> MNQIWLKVCAASDMQPGTIRRVNRVGA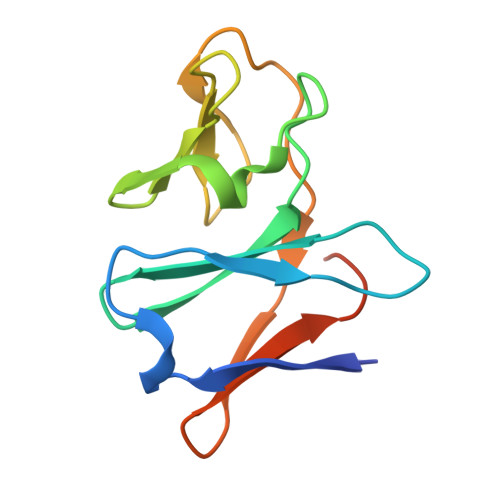APLAVYRVGDQFYATEDTCTHGIASLSEGTLDGDVIECPFHGGAFNVCTGMPASSPCTVPLGVFEVEVKEGEVYVAGEKKLEHHHHHH> GPDGMAALSLPLPISAGRGYAPAFTLNYNSGAGNSPFGLGWDCNVMTIRRRTHFGVPHYDETDTFLGPEGEVLVVADQPRDESTLQGINLGATFTVTGYRSRLESHFSRLEYWQPKTTGKTDFWLIYSPDGQVHLLGKSPQARISNPSQTTQTAQWLLEASVSSRGEQIYYQYRAEDDTGCEADEITHHLQATAQRYLHIVYYGNRTASETLPGLDGSAPSQADWLFYLVFDYGERSNNLKTPPAFSTTGSWLCRQDRFSRYEYGFEIRTRRLCRQVLMYHHLQALDSKITEHNGPTLVSRLILNYDESAIASTLVFVRRVGHEQDGNVVTLPPLELAYQDFSPRHHAHWQPMDVLANFNAIQRWQLVDLKGEGLPGLLYQDKGAWWYRSAQRLGEIGSDAVTWEKMQPLSVIPSLQSNASLVDINGDGQLDWVITGPGLRGYHSQRPDGSWTRFTPLNALPVEYTHPRAQLADLMGAGLSDLVLIGPKSVRLYANTRDGFAKGKDVVQSGDITLPVPGADPRKLVAFSDVLGSGQAHLVEVSATKVTCWPNLGRGRFGQPITLPGFSQPATEFNPAQVYLADLDGSGPTDLIYVHTNRLDIFLNKSGNGFAEPVTLRFPEGLRFDHTCQLQMADVQGLGVASLILSVPHMSPHHWRCDLTNMKPWLLNEMNNNMGVHHTLRYRSSSQFWLDEKAAALTTGQTPVCYLPFPIHTLWQTETEDEISGNKLVTTLRYARGAWDGREREFRGFGYVEQTDSHQLAQGNAPERTPPALTKNWYATGLPVIDNALSTEYWRDDQAFAGFSPRFTTWQDNKDVPLTPEDDNSRYWFNRALKGQLLRSELYGLDDSTNKHVPYTVTEFRSQVRRLQHTDSRYPVLWSSVVESRNYHYERIASDPQCSQNITLSSDRFGQPLKQLSVQYPRRQQPAINLYPDTLPDKLLANSYDDQQRQLRLTYQQSSWHHLTNNTVRVLGLPDSTRSDIFTYVAENVPAGGLNLELLSDKNSLIADDKPREYLGQQKTAYTDGQNTTPLQTPTRQALIAFTETTVFNQSTLSAFNGSIPSDKLSTTLEQAGYQQTNYLFPRTGEDKVWVAHHGYTDYGTAAQFWRPQKQSNTQLTGKITLIWDANYCVVVQTRDAAGLTTSAKYDWRFLTPVQLTDINDNQHLITLDALGRPITLRFWGTENGKMTGYSSPEKASFSPPSDVNAAIELKKPLPVAQCQVYAPESWMPVLSQKTFNRLAEQDWQKLYNARIITEDGRICTLAYRRWVQSQKAIPQLISLLNNGPRLPPHSLTLTTDRYDHDPEQQIRQQVVFSDGFGRLLQAAARHEAGMARQRNEDGSLIINVQHTENRWAVTGRTEYDNKGQPIRTYQPYFLNDWRYVSNDSARQEKEAYADTHVYDPIGREIKVITAKGWFRRTLFTPWFTVNEDENDTAAEVKKIDPKLYQKTPTVSVYDNRGLIIRNIDFHRTTANGDPDTRITRHQYDIHGHLNQSIDPRLYEAKQTNNTIKPNFLWQYDLTGNPLCTESIDAGRTVTLNDIEGRPLLTVTATGVIQTRQYETSSLPGRLLSVAEQTPEEKTSRITERLIWAGNTEAEKDHNLAGQCVRHYDTAGVTRLESLSLTGTVLSQSSQLLIDTQEANWTGDNETVWQNMLADDIYTTLSTFDATGALLTQTDAKGNIQRLAYDVAGQLNGSWLTLKGQTEQVIIKSLTYSAAGQKLREEHGNDVITEYSYEPETQRLIGIKTRRPSDTKVLQDLRYEYDPVGNVISIRNDAEATRFWHNQKVMPENTYTYDSLYQLISATGREMANIGQQSHQFPSPALPSDNNTYTNYTRTYTYDRGGNLTKIQHSSPATQNNYTTNITVSNRSNRAVLSTLTEDPAQVDALFDAGGHQNTLISGQNLNWNTRGELQQVTLVKRDKGANDDREWYRYSGDGRRMLKINEQQASNNAQTQRVTYLPNLELRLTQNSTATTEDLQVITVGEAGRAQVRVLHWESGKPEDIDNNQLRYSYDNLIGSSQLELDSEGQIISEEEYYPYGGTALWAARNQTEASYKTIRYSGKERDATGLYYYGYRYYQPWIGRWLSSDPAGTIDGLNLYRMVRNNPVTLLDPDGLNVFDEAILAALEP

Tc toxins consist of three components: TcA, TcB, and TcC. We therefore chose TcdB2-TccC3 to function as a cocoon scaffold for translocation of other cargo proteins, which are not components of the Tc toxin system.

Similarly to TccC3HVR in the TcB-TcC(WT) cocoon, Cdc42 is not structured inside the cocoon. However, we found an ordered electron density in close spatial proximity to the β-propeller domain, which corresponds to an α-helix not present in other TcB-TcC structures obtained so far. Importantly, the helix is attached to the TcB protein in an orientation perpendicular to that expected from natural translocation, and its amphipathic nature facilitates interaction with a hydrophobic pocket on the inner surface of the cocoon. The side chains of F169, I173, L177, and P179 are rigidly oriented toward the hydrophobic cleft, where they are in close contact with L39, L41, P42, L366, L368, M702, N704, V708, H710, L1203, and F1349 of the cocoon. Interestingly, the affinity of the Cdc42 α-helix for this part of the cocoon is strong enough to displace the N-terminus of TcB, which resides at this position in TcB-TcC(WT). The N-terminus of TcB-TcC-Cdc42 is correspondingly not resolved, indicating that it protrudes into the cocoon lumen. The tight attachment of Cdc42 via its C-terminus in close spatial proximity to the TcB gatekeeper domain16 could help this construct to form a holotoxin with high affinity comparable to the constructs with larger cargos, despite Cdc42 being at the lower limit of the cargo size prerequisite. The tight association of the C-terminal α-helix to the cocoon results in Cdc42 translocation arrest already at an early stage.>HMLRPVETPTREIKKLDGLWAFSLDRENCGIDQRWWESALQESRAIAVPGSFNDQFADADIRNYAGNVWYQREVFIPKGWAGQRIVLRFDAVTHYGKVWVNNQEVMEHQGGYTPFEADVTPYVIAGKSVRITVCVNNELNWQTIPPGMVITDENGKKKQSYFHDFFNYAGIHRSVMLYTTPNTWVDDITVVTHVAQDCNHASVDWQVVANGDVSVELRDADQQVVATGQGTSGTLQVVNPHLWQPGEGYLYELCVTAKSQTECDIYPLRVGIRSVAVKGEQFLINHKPFYFTGFGRHEDADLRGKGFDNVLMVHDHALMDWIGANSYRTSHYPYAEEMLDWADEHGIVVIDETAAVGFNLSLGIGFEAGNKPKELYSEEAVNGETQQAHLQAIKELIARDKNHPSVVMWSIANEPDTRPQGAREYFAPLAEATRKLDPTRPITCVNVMFCDAHTDTISDLFDVLCLNRYYGWYVQSGDLETAEKVLEKELLAWQEKLHQPIIITEYGVDTLAGLHSMYTDMWSEEYQCAWLDMYHRVFDRVSAVVGEQVWNFADFATSQGILRVGGNKKGIFTRDRKPKSAAFLLQKRWTGMNFGEKPQQGGKQ[2x]

However, intestinal bacterial GUSs cleave the attached glucuronic acid for use as a carbon source, allowing potentially toxic compounds to re-enter the enterohepatic circulation. However, microflora-encoding β-glucuronidases (GUSs) are notorious for reversing the glucuronidation to release SN-38 in the intestinal lumen and thus represent the major cause of undesirable effects. GUS contains a deep enzyme active site (the two catalytic glutamates lie ~12 Å below the protein surface). To understand the underlying structural basis, we prepared C6-propyl, -hexyl, and -nonyl UIFGs (2–4, respectively) and resolved the eight X-ray crystal structures of 1–4 bound to EcGUS or Bifidobacterium dentium GUS (BdGUS).

Though less potent for LgGUS and BdGUS, 4 still inhibited these two GUSs in the sub-micromolar range (Ki = 270 and 440 nM, respectively) and was selective for the two bacterial GUSs (390- and 240-fold more potent than for HsGUS, respectively). Likewise, C6-hexyl UIFG also was 1770-fold more potent for inhibiting EcGUS than HsGUS. Furthermore, EcGUS contains a narrower aglycone-binding site than LgGUS and BdGUS. Taking the comparison between EcGUS and HsGUS as an example, the aglycone-binding site of EcGUS is surrounded by five hydrophobic residues, namely Phe365, Leu361, Val446, Met447, and Phe448, which are located in loops 3 and 5, whereas the site of HsGUS is surrounded by Ser485loop 5, Tyr505loop 6, His509loop 6, and Thr599loop 8. The alkyl substituent of the inhibitors therefore facilitated an increase in hydrophobic contacts with nonpolar residues of loops 3 and 5 in EcGUS, e.g., such as Leu361, Phe365 in loop 3, and Val446, Met447, and Phe448 in loop 5. Interestingly, owing to the longer alkyl chains of 3 and 4, Phe448 rotated outward in EcGUS/3 and EcGUS/4 and thus increased the hydrophobic contact area. This additional hydrophobic interaction might have compensated for the binding energy loss owing to the absence of the water-mediated H-bond network, leading to the observed lower Ki values of 2–4 for EcGUS compared with other GUSs. Similar to the previous trend, the entropy contribution of 3 and 4 increased with the length of alkyl chain (–TΔΔS2–3 = –1.32 kcal mol−1 and –TΔΔS2–4 = −1.34 kcal mol−1 for EcGUS), while the enthalpy contribution decreased (ΔΔH2–3 = +0.04 kcal mol−1 and ΔΔH2–4 = +0.99 kcal mol−1 for EcGUS).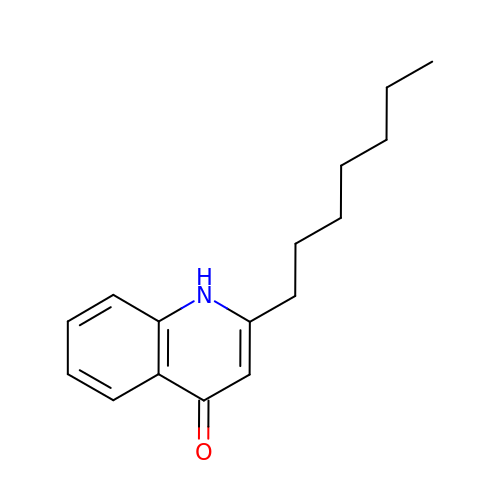2-heptyl-1~{H}-quinolin-4-one | C16 H21 N O | UYRHHBXYXSYGHA-UHFFFAOYSA-N>GSGMMAEPDPSHPLETQAGKVQEAQDSDSDSEGGAAGGEADMDFLRNLFSQTLSLGSQKERLLDELTLEGVARYMQSERCRRVICLVGAGISTSAGIPDFRSPSTGLYDNLEKYHLPYPEAIFEISYFKKHPEPFFALAKELYPGQFKPTICHYFMRLLKDKGLLLRCYTQNIDTLERIAGLEQEDLVEAHGTFYTSHCVSASCRHEYPLSWMKEKIFSEVTPKCEDCQSLVKPDIVFFGESLP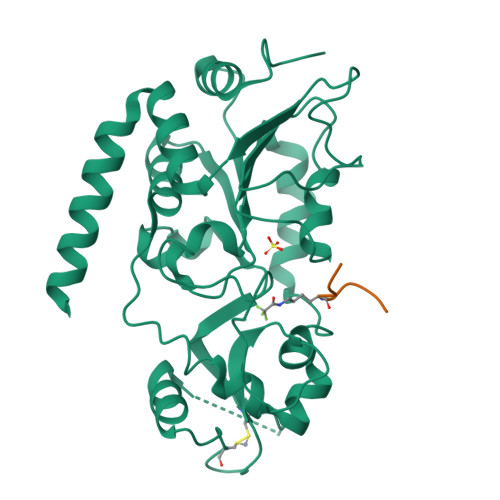ARFFSCMQSDFLKVDLLLVMGTSLQVQPFASLISKAPLSTPRLLINKEKAGQSDPFLGMIMGLGGGMDFDSKKAYRDVAWLGECDQGCLALAELLGWKKELEDLVRREHASIDAQS[2x];>[2x]LTGEFEKKYVATL>[2x]GAMARKELSSLEELFRHYGVRYMTLTKMVEMGFTVNTLVNMTEQELDDVIRTLVDIYRVDLLVGEKYGIKSAVRAEKRRLDELERKKLDLFVDVDGKRKADENALDTLSQ

Here we focus on LEAFY (LFY), a plant-specific TF essential for flower development. LFY is one of the few master regulators of flower development, as it integrates environmental and endogenous signals to orchestrate the whole floral network11121314. Structure–function studies have demonstrated that LFY binds semi-palindromic 19-bp DNA elements through its highly conserved C-terminal DBD, a unique helix-turn-helix fold that by itself dimerizes on DNA. In addition to its well-characterized DBD, LFY possesses a second conserved domain at its amino terminus (LFY-N).

After heterologously overexpressing LFY-N domains from different plant species, we were able to determine the crystal structure for GbLFY-N from the gymnosperm Ginkgo biloba at 2.3 Å resolution. This structure showed that the GbLFY-N monomer is made up of five α-helices separated by four loops. Comparison against the Protein Data Bank revealed a strong structural similarity with the SAM, also called Pointed domain28, a resemblance that could not be predicted from LFY-N sequences. Some SAM domains are able to self-associate as oligomers through the so-called mid-loop (ML) and end-helix (EH) surfaces. GbLFY-SAM appears to belong to this class: in the crystal, it forms a head-to-tail polymer with monomers contacting their neighbours through two polar surfaces. The ML surface comprises negative and polar residues, including T72, T75 and E83, which interact with the positively charged EH surface through hydrogen bonds and salt bridges, in particular via R112 and R116 (residue numbering refers to LFY from A. thaliana—AtLFY—sequence). Size-exclusion chromatography coupled to multi-angle laser light scattering (SEC-MALLS) showed that the WT GbLFY-SAM domain formed oligomers of variable size in solution, depending on protein concentration, containing up to eight monomers. In comparison, all mutations affecting the interaction interface completely abolished LFY oligomerization and GbLFY-SAMTE, GbLFY-SAMRE and GbLFY-SAMTERE proteins were found to be exclusively monomeric. However, when mixed at an equimolar ratio, the GbLFY-SAMTE and GbLFY-SAMRE single-face mutants retained the ability to interact, forming a GbLFY-SAM[RE+TE] dimer, thus showing that the different mutations did not alter the overall fold of the SAM domain, and that single face mutant proteins still displayed one functional interaction surface. These results further showed that the head-to-tail arrangement observed in the crystal structure reflects the state of LFY-SAM in solution, which forms an oligomer of limited size in the conditions of this study. Our results demonstrate that LFY-N is a Sterile Alpha Motif (SAM) domain that mediates LFY oligomerization.> MKTYEVGALLEAANQRDTKKVKEILQDTTYQVDEVDTEGNTPLNIAVHNNDIEIAKALIDRGADINLQNSISDSPYLY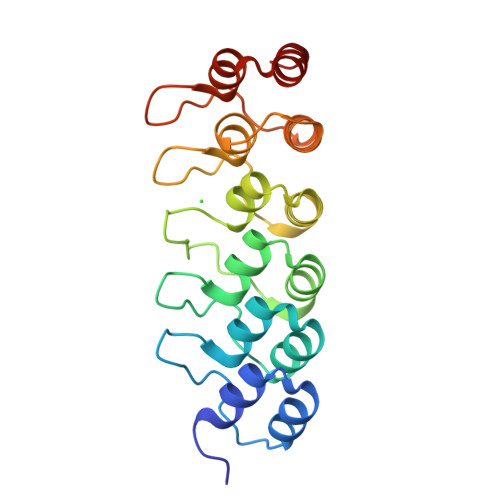AGAQGRTEILAYMLKHATPDLNKHNRYGGNALIPAAEKGHIDNVKLLLEDGREDIDFQNDFGYTALIEAVGLREGNQLYQDIVKLLMENGADQSIKDNSGRTAMDYANQKGYTEISKILAQYN> MFLLAVYFLFFSAIANGFFGRYLGVRGSQLLGPSALFLALL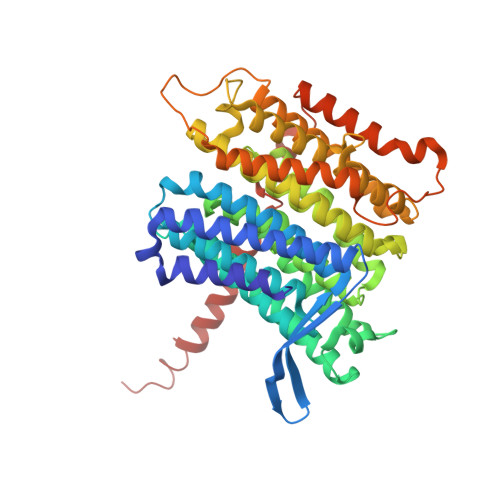CSGTIFYEVCIQGCSTNIKLFENFVYSNELNVSASFLYDPLAATMTLTVVWISCAVHAYQNLYMRGDGSQTLFTSYLSAFTGFMLILVAGQNLVMLFIGWEGIGVCSYLLIGYYGSRVSAVKSANKSLIVNKISDGFLLGSMLYLWFYTGSFSYCSLATFQIPDVVSILVLLGAIGKSSQLFFHVWLADAMEGPTPVSALIHAATLVTAGIYVLCKLNLHSQSAVGILGAATALMGGLFGLAANDLKRVIAFSTCSQLGYMMAVLSTCDDGADFAMGHLVSHAGFKATLFLSAGLSIAKENNNFLNRYGSRQGSPTLSFATTIASLNLLGFPELGGFYSKESILNNAYINQGVSIILTLATFLTAFYTSKVLAQLYLFPYGNGRQQKSFDIDATTLICFGLLLSEMLLRIFTGSSLSQNMTTNLPAHIKNLPFWVALSGALSGLATTNLFSSNFMRFFGNRGGFDVFYARKCSNVFYHNAYVSYTLLDRGFLKLY> MAAQGFLLIATFLLVLMVLARPLGSGLARLINDIPLPGTTGVERVLFRALGVSDREMNWKQYLCAILGLNMLGLAVLFFMLLGQHYLPLNPQQLPGLSWDLALNTAVSFVTNTNWQSYSGETTLSYFSQMAGLTVQNFLSAASGIAVIFALIRAFTRQSMSTLGNAWVDLLRITLWVLVPVALLIALFFIQQGALQNFLPYQAVNTVEGAQQLLPMGPVASQEAIKMLGTNGGGFFNANSSHPFENPTALTNFVQMLAIFLIPTALCFAFGEVMGDRRQGRMLLWAMSVIFVICVGVVMWAEVQGNPHLLALGTDSSINMEGKESRFGVLVSSLFAVVTTAASCGAVIAMHDSFTALGGMVPMWLMQIGEVVFGGVGSGLYGMMLFVLLAVFIAGLMIGRTPEYLGKKIDVREMKLTALAILVTPTLVLMGAALAMMTDAGRSAMLNPGPHGFSEVLYAVSSAANNNGSAFAGLSANSPFWNCLLAFCMFVGRFGVIIPVMAIAGSLVSKKSQAASSGTLPTHGPLFVGLLIGTVLLVGALTFIPALALGPVAEYLS;> MSRKQLALFEPTLVVQALKEAVKKLNPQAQWRNPVMFIVWIGSLLTTCISIAMASGAMPGNALFSAAISGWLWITVLFANFAEALAEGRSKAQANSLKGVKKTAFARKLREPKYGAAADKVPADQLRKGDIVLVEAGDIIPCDGEVIEGGASVDESAITGEAAPVIRESGGDFASVTGGTRILSDWLVIECSVNPGETFLDRMIAMVEGAQRRKTPNEIALTILLIALTIVFLLATATLWPFSAWGGNAVSVTVLVALLVCLIPTTIGG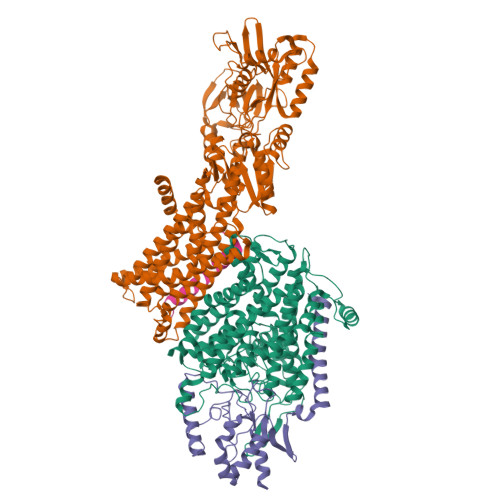LLSAIGVAGMSRMLGANVIATSGRAVEAAGDVDVLLLDKTGTITLGNRQASEFIPAQGVDEKTLADAAQLASLADETPEGRSIVILAKQRFNLRERDVQSLHATFVPFTAQSRMSGINIDNRMIRKGSVDAIRRHVEANGGHFPTDVDQKVDQVARQGATPLVVVEGSRVLGVIALKDIVKGGIKERFAQLRKMGIKTVMITGDNRLTAAAIAAEAGVDDFLAEATPEAKLALIRQYQAEGRLVAMTGDGTNDAPALAQADVAVAMNSGTQAAKEAGNMVDLDSNPTKLIEVVHIGKQMLMTRGSLTTFSIANDVAKYFAIIPAAFAATYPQLNALNIMCLHSPDSAILSAVIFNALIIVFLIPLALKGVSYKPLTASAMLRRNLWIYGLGGLLVPFIGIKVIDLLLTVCGLV;> MSGLRPALSTFIFLLLITGGVYPLLTTVLGQWWFPWQANGSLIREGDTVRGSALIGQNFTGNGYFHGRPSATAEMPYNPQASGGSNLAVSNPELDKLIAARVAALRAANPDASASVPVELVTASASGLDNNITPQAAAWQIPRVAKARNLSVEQLTQLIAKYSQQPLVKYIGQPVVNIVELNLALDKLDE;> MSAGVITGVLLVFLLLGYLVYALINAE Macrolide resistance is abundant in pathogenic bacteria, and is most often the result of GTP-dependent macrolide kinases (Mph), ribosomal methyltransferases, or efflux pumps. Mph enzymes inactivate macrolides by phosphorylating the 2′-OH of the essential dimethylamino sugar, preventing it from binding the ribosome, and providing the chemical rationale for the resistance phenotype. Mph enzymes are therefore adaptable resistance enzymes with complex evolutionary paths.

In contrast to previous reports, we found that MphB confers resistance to all macrolides tested, and inactivates both telithromycin and azithromycin. Using tandem mass spectrometry, we also confirmed that MphB phosphorylates the desosamine 2′-OH of erythromycin. Moreover, MphB modifies macrolides with efficiencies comparable to other Mphs (kcat/Km 104–106), and the Km for C3 cladinose macrolides is 19–69× lower than MphI. While preparing this manuscript, crystal structures of MphA and MphB were reported in complex with various macrolides, which we have included in our analysis of substrate specificity. While the MphA, MphB, and MphH structures are very similar, we observed structural distinctions in all three enzymes that localized to the (a) NPL, (b) β-hairpin insert, and (c) multiple residues in the macrolide-binding cleft. As we observed in MphH, the NPL, and β-hairpin regions of both MphA and MphB adopt different conformations with macrolide binding.

> MSKDIKQVIEIAKKHNLFLKEETIQFNESGLDFQAVFAQDNNGIDWVLRLPRREDVMPRTKVEKQALDLVNKYAISFQAPNWIIYTEELIAYKKLDGVPAGTIDHNIGNYIWEIDINNVPELFHKSLGRVLAELHSIPSNKAAALDLVVHTPEEARMSMKQRMDAVRAKFGVGENLWNRWQAWLNDDDMWPKKTGLIHGDVHAGHTMIDKDANVTGLIDWTEAKVTDVSHDFIFNYRAFGEEGLEALILAYKEIGGYYWPKMKEHIIELNAAYPVSIAEFALVSGIEEYEQMAKEALEVQGS>[6x]GTHMKEPRNVRLTFADIELDEETHEVWKAGQPVSLSPT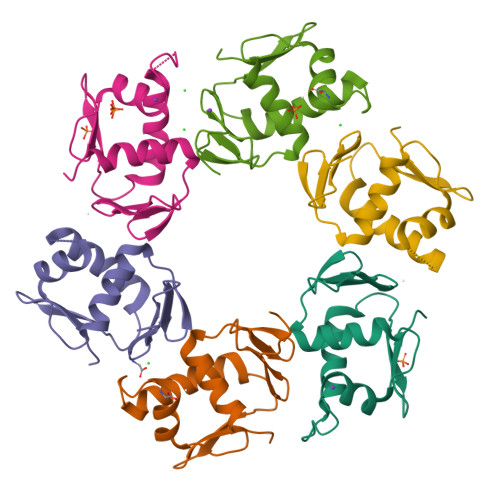EFTLLRYFVINAGTVLSKPKILDHVWRYDFGGDVNVVESYVSYLRRKIDTGEKRLLHTLRGVGYVLREPRKL> MSALCWGRGAAGLKRALRPCGRPGLPGKEGTAGGVCGPRRSSSASPQEQDQDRRKDWGHVELLEVLQARVRQLQAESVSEVVVNRVDVARLPECGSGDGSLQPPRKVQMGAKDATPVPCGRWAKILEKDKRTQQMRMQRLKAKLQMPFQSGEFKALTRRLQVEPRLLSKQMAGCLEDCTRQAPESPWEEQLARLLQEAPGKLSLDVEQAPSGQHSQAQLSGQQQRLLAFFKCCLLTDQLPLAHHLLVVHHGQRQKRKLLTLDMYNAVMLGWARQGAFKELVYVLFMVKDAGLTPDLLSYAAALQCMGRQDQDAGTIERCLEQMSQEGLKLQALFTAVLLSEEDRATVLKAVHKVKPTFSLPPQLPPPVNTSKLLRDVYAKDGRVSYPKLHLPLKTLQCLFEKQL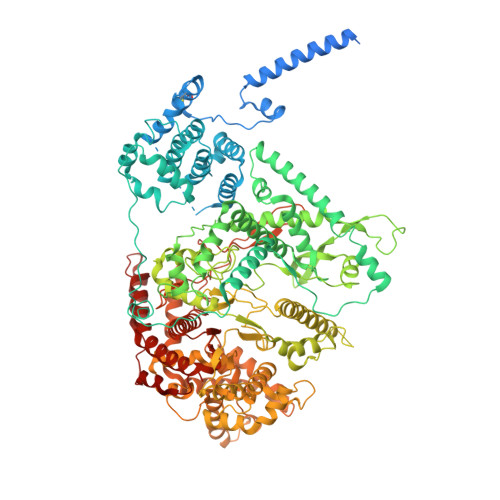HMELASRVCVVSVEKPTLPSKEVKHARKTLKTLRDQWEKALCRALRETKNRLEREVYEGRFSLYPFLCLLDEREVVRMLLQVLQALPAQGESFTTLARELSARTFSRHVVQRQRVSGQVQALQNHYRKYLCLLASDAEVPEPCLPRQYWEELGAPEALREQPWPLPVQMELGKLLAEMLVQATQMPCSLDKPHRSSRLVPVLYHVYSFRNVQQIGILKPHPAYVQLLEKAAEPTLTFEAVDVPMLCPPLPWTSPHSGAFLLSPTKLMRTVEGATQHQELLETCPPTALHGALDALTQLGNCAWRVNGRVLDLVLQLFQAKGCPQLGVPAPPSEAPQPPEAHLPHSAAPARKAELRRELAHCQKVAREMHSLRAEALYRLSLAQHLRDRVFWLPHNMDFRGRTYPCPPHFNHLGSDVARALLEFAQGRPLGPHGLDWLKIHLVNLTGLKKREPLRKRLAFAEEVMDDILDSADQPLTGRKWWMGAEEPWQTLACCMEVANAVRASDPAAYVSHLPVHQDGSCNGLQHYAALGRDSVGAASVNLEPSDVPQDVYSGVAAQVEVFRRQDAQRGMRVAQVLEGFITRKVVKQTVMTVVYGVTRYGGRLQIEKRLRELSDFPQEFVWEASHYLVRQVFKSLQEMFSGTRAIQHWLTESARLISHMGSVVEWVTPLGVPVIQPYRLDSKVKQIGGGIQSITYTHNGDISRKPNTRKQKNGFPPNFIHSLDSSHMMLTALHCYRKGLTFVSVHDCYWTHAADVSVMNQVCREQFVRLHSEPILQDLSRFLVKRFCSEPQKILEASQLKETLQAVPKPGAFDLEQVKRSTYFFS>MYTIARIATRAAVSQGSQAYLRPVSSAVLSQKVIVEAPVATQARSLQTSAVQRDIDSAAKFIGAGAATVGVAGSGAGIGSVFGSLIIGYARNPSLKQQLFSYAILGFALSEAMGLFCLMMAFLLLFAF[8x];> MFGRTSVLVLSQCNAAEQVRGMATLKAVSIRLKSVKNIQKITQSMKMVSAAKYTKAERELRVAKPYGQGAMKFYEKTELKGKEEKPSQLIIAISSDRGLCGAVHSSVGRQLKADLAANPDTMVICVGDKIRNILQRLYGNNLAMVCNDFGRRPPVFEDATKVARAVLESGMEFTNGKIVYNAFRSVVSFRTTDIPVFSKNAIESADSIAAYDSLDSDVIQSYVEYSLASLIYYTMKENATSEQSSRMTAMDNASKNAGEMIDKLTMTFNRTRQAVITRELIEIISGASAL;> MVSLTGDVSTVVGPTEVDSAEVGFADVSSAWDNQMAFTFAAPSQVFYNNANIRQVDVPSFSGSFGILPAHVATLAVLKPGVVTVYQEDGSTKKYFVSSGTVTVNDDSSVQVLAEEAVPVENLDLQAARDILSKAQSDVTSAGADMLKLAEGQIAVEVGEALVKAAEGQL;> VRSNFASISGSGRRGRHVDFGASVDFEVHMMRRALKPELRNEAIKREESLLKVTPWKDGKPVKAAQ;> MLSRIAVQSARPIAALQSVRPVQTSSTKTSEVASASVAPVVQFKGPNEGVERDHVGFPRPLRPVNPGKVRVGFVPEEWFTFFYNKTGVTGPYVLGAGALTFLLSKEIYVVEHEFYTGVAIAIMGTYGVKKFGKQIADYADKGIGEIEQSFKEYQDSSKIGFEEAITLEERAQKSAEAQIMLFQAKRENVQFQLEAAYRARLHHVNNEIKKRLDYHLETERAQRQIKQKNMVDWIVRNVMKSITPEQERLMLSKCISDLKAMSIKA;> MASKRIARSSIDWAKMAESVPESQKAMYNQFKAKSDGYIRKALSYPEQPSPINWEHYRKSLTNPAMVDAFKKQYEALKVPYPEDKVSSQIDAQEAEAKKEITKFIQESRGRIENYKAELGKLGQMIPFEHMTLEDFFEAFPEKVLNPDPPSPNVKKKPFKNNSWHLIQKIPNHFGLILKKTLWNSKRRNSGNLEMNTIKSILLLDIIFKSFIGIKMCKL;> MMASLFSVFDPTSSFLSNWLSMLIPLLFMVMSFWLIPSRPQFLAKSVLMGLNREMSLLMGPASFGANILVIALFLFILFNNFIGLFPYIFTATSHLAVTLSLAVPLWISFILYTWIKETTNALAHLVPLGTPAPLMPFMVLMEIISNMIRPITLSVRLAANMIAGHLLLTLLGAQGTLENLYVTSIVVFSQIILLMLEFSVAIIQSYVFMTLMTLYASE;> MPQMMPLPWIMVFLVSMALLWAIMTMVFFLYQPRSVSSAKGFSDRTVYLNWKW;> MGFGDYPAEYNPKVHGPYDPARFYGKADVPLGQVKLGELSQWLGRRNKNPQAVAAAVSRGWWRWQHKYVLPRKGGIAPYIQLIVGCSIFFYAINYGKMVAHRQRKYHCRKTHSISHSNI;> MSALAKKIATSGPVVLKNTIAVTRPKLATFLKYAKVELTPPGPADVPKIQEGIQNLIHSAKTGKWKQVSVREAWLNTLIVTEIAMWFFVGECIGKGSVIGYRV;> MSFAPPVNVSPLIRAGRYGALVVGIVYGSYRFGSLQKRENEWRVEEARRKVIRDALNAENKAKATREEMLYLAKETGVKVPENF

ATP synthase is a unique molecular engine that uses the rotation of its subunits to perform the catalytic reaction of ATP synthesis and hydrolysis. Unlike in mammals, mitochondria of the crustacean Artemia franciscana have the ability to accumulate large amounts of Ca2+ without undergoing the mPT. Here, we performed structural and functional analysis of A. franciscana ATP synthase to study the molecular mechanism of mPTP inhibition in this organism. We found that the channel formed by the A. franciscana ATP synthase dwells predominantly in its inactive state and is insensitive to Ca2+, in contrast to porcine heart ATP synthase.

The local refined map for FO at state 1 had a resolution of 3.3 Å. The FO domain of A. franciscana has the same subunit composition and overall structure as the mammalian ATP synthases. It consists of the c8-ring and a-subunit (subunit 6 or ATP6) that form the proton translocation pathway, as well as subunits 6.8PL, subunit 8 (ATP8), e, f, and g. Two native cardiolipin molecules (CDL1 and CDL2) were found in the A. franciscana FO domain between subunits a, b, f, and g. CDL1 is located between the subunits a, b, and f, interacting with the α-helical domains aH3, aH6, cH1, bH3, and fH4. The second cardiolipin molecule, CDL2, was found between the subunits b, f, and g and interacts with the helical domains fH1, fH3, fH4, bH1, bH2, and gH3. Furthermore, a stronger density of the e-subunit C-terminus was observed in the A. franciscana maps in contrast to mammalian structures. In addition, the C-terminus of the A. franciscana e-subunit has a different conformation; it is more curved and extends towards the c-ring lumen compared with the ovine ATP synthase. The distances are suggestive of the following interactions between subunit e and the c-ring: Salt bridges between eK61 and cD1 residues, and eK79 and cD1, and a hydrogen bond between eY71 and cD1 may form in A. franciscana FO. The residues eK79 and eY71 may also interact with the c-ring lipids.>[2x]MAHHHHHHVGTFENITAAPADPILGLADLFRADERPGKVDLGVGVYKDETGKTPVMTSVKKAEQYL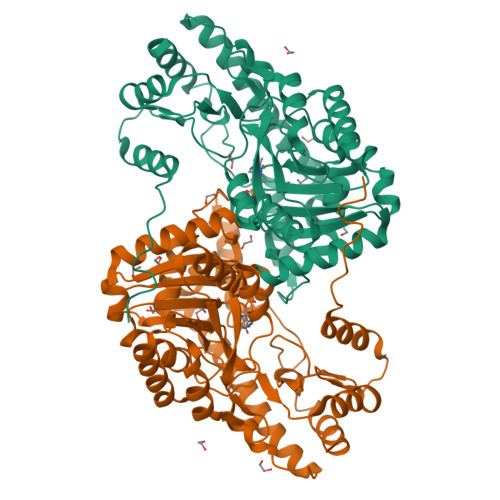LENETTKTYLGLDGLPEFGRCTQELLFGKGSALINDKRARTAQTPGGSGALRVAADFLAKNTSVKRVWVSNPTWPNHKAIFNSAGLEVREYAYYDAENHTLDFDALINSLNEAQAGDVVLFHGCCHNPTGADPTLEQWQTLAQLSVEKGWLPLIDIAYQGFGRGLEEDAEGLRAFAAMHKELIVASSCSKNFGLYNERVGACTLVAADSETVDRAFSQMKAAIRANYSSPPAHGASVVATILSNDALRAIWEQELTDMRQRIQRMRQLFVNTLQEKGANRDFSFIIKQNGMFSFSGLTKEQVLRLREEFGVYAVASGRINVAGMTPDNMAPLCEAIVAVL>[2x]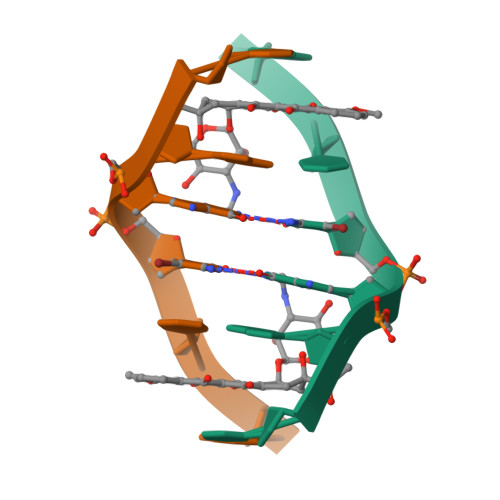CGGCCG>[2x]MSALHALVQGPATAAAPRLTEPERAVVQRELDELARGGYTGPLLESLRKLAAAVPERLYDDSARVLLRMHEIAGSGNYQSNLSSLPLVRACFDLGLVPEDGPGPAELIVGRGHIAPAFYAEHYVRGTFPFAPLATLHQGGLTGVVHQDLGFTNTMRYSLGVGVAQAVSLAWELTRRGEDRK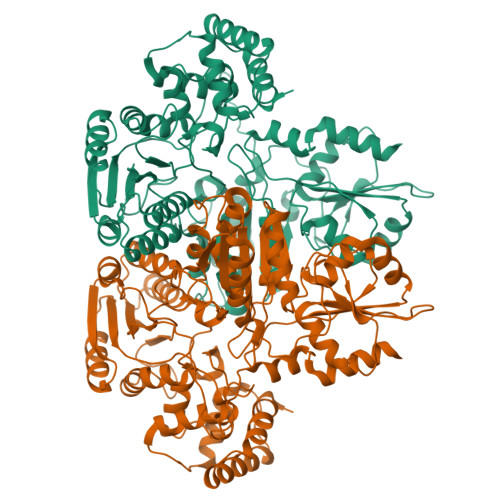VVCLAGDGELQEGVVFECLRFAHEADLKNLILVVDTNDKGIEPLLKPLSRGYLASYLDRVEEVDGLDTATVRDSLGALLAAPTSAALVCRTRKGDHSFKPATTAPATAPRPAKVSFANTSGAALAAYRERTGRELAVFTADMAARFGLRDKVPYTNTGLAETLSLGLTLSLPEETVKVVATDAMYYMDSLSMLTEATTSVRNLLVLAGRSWGAWGGAHNATNLLGQLLHTRVYEPVTAAEFAACLDRLDRHPDTTHVVSTVDAKFDPPPADCAGDVDGGTWLTPPGDGPPRAAVVTFGYAGVLVAEANRDLGVPHLHCAALEPDLDARTLAQLGACEDLLTVEYNGVHGGFGERLRTTYLLPARVHGVRQDIANRVHDRQLRLHGMGPEQLDALLRGLTG Phytochromes (Phys) are a divergent cohort of bili-proteins that detect light through reversible interconversion between dark-adapted Pr and photoactivated Pfr states. Here, we present models of both states for a dimeric Phy with histidine kinase (HK) activity from the proteobacterium Pseudomonas syringae, which were built from high-resolution cryo-EM maps (2.8–3.4-Å) of the photosensory module (PSM) and its following signaling (S) helix together with lower resolution maps for the downstream output region augmented by RoseTTAFold and AlphaFold structural predictions. Pr/Pfr comparisons show that bilin phototransformation alters PSM architecture culminating in a scissoring motion of the paired S-helices linking the PSMs to the HK bidomains that ends in reorientation of the paired catalytic ATPase modules relative to the phosphoacceptor histidines. This action apparently primes autophosphorylation enroute to phosphotransfer to the cognate DNA-binding response regulator AlgB which drives quorum-sensing behavior through transient association with the photoreceptor.

We then defined by cryo-EM a 3D model of the full-length PsBphP1 dimer as Pfr by analyzing red light-irradiated samples. Here, 4,796,622 particle images were extracted and winnowed down to 1,029,141 after 2D classification, which revealed three similar but distinct EM density maps representing unique structural conformations of the photoactivated photoreceptor. Two maps resolved to 3.1- and 3.0-Å were dimeric head-to-head arrangements of the PSM with only short S-helix extensions visible beyond the PHY domains. The PAS-GAF regions were intimately connected in the dimer like those in Pr while the paired PHY domains were either moderately or strongly splayed (designated “medial” and “splayed”, respectively). Both the BV and hairpin conformations matched previous views of Phys as Pfr14,15,22,25. Much like the high-resolution Pr EM density map, these two Pfr maps lacked the HK bidomains and much of the S-helices presumably due to high mobility. Importantly, the PSM regions of all three maps (DoD, medial, and splayed) allowed unambiguous modeling of both protomers as Pfr as judged by sufficiently resolved ZZEssa conformations of the bilins that aligned well for all three maps except for slightly different tilts of the D rings and by the presence of obvious α-helical hairpins, which are both signatures of this spectral state. The Pfr maps presented an even more complicated picture where the three divergent conformational states seen here (DoD, medial, and splayed) implied that the S-helices become more pliable and possibly even allow dissociation of the HK bidomains as inferred by the conformation of the “splayed” Pfr model. Although the data for the DoD form provided structural appreciations for positioning of the HK bidomains, similar data for the splayed and medial forms of Pfr were absent, suggesting that the HK bidomain positioning is highly dynamic in these states.

>[2x]GMSQLDKDAFEVLLANCADEPIQFPGAIQPHGLLFTLKEPELTILQVSANVQSVLGKVPDQLAGQTLDCVLGAGWAEVIRSTSANDSLVDVPRLLMSVEGVEFEALLHRSQEALVLELEIQDKAAQAISYSERTGNMGRMLRQLHAAADLQTLYEVSVREIQRMTGYDRVLIYRFEEEGHGQVIAEASAPAMELFNGLFFPASDIPEQARELYRRNWLRIIPDANYTPVPLVPQLRPDTQQQLDLSFSTLRSVSPIHCQYMKNMGVLSSMSVSLIQGGKLWGLISCGHRTPLYVSHELRSACQAIGQVLSLQISAMEALEVSRQRETKIQTLQQLHQMMATSDTDVFDGLAQQPQLLMDLVGATGVAIIEDRQTHCYGNCPEPSDIRALHTWMMAGGEPVYASHHLSSVYPPGEAYQTLASGVLAMSLPKPVDNGVIWFRPEVKQSVQWSGDPNKPLNLDASDNTLRLQPRTSFEIWKVEMTGIATKWSHGDVFAANDLRRSALENDLARQVSKEQQAVRARDELVAVVSHDLRNPMTVISMLCGMMQKSFSSDGPHTSRRISTAIDTMQQAASRMNVLLEDLLDTSKIEAGRYTITPQPLEVSQIFEEAYTLLAPLAMDKSIEISFNAEPDIKVNADPERLFQVLSNLIGNAIKFTPKLGRIGVAAMSNGDEVVFTVRDSGEGIPPEQLPHIFERYWTVKEGNPTGTGLGLYISQGIIKAHGGELAAQSQVGHGSEFRFTVPIAH> ASMKNCVIVSAVRTAIGSFNGSLASTSAIDLGATVIKAAIERAKIDSQ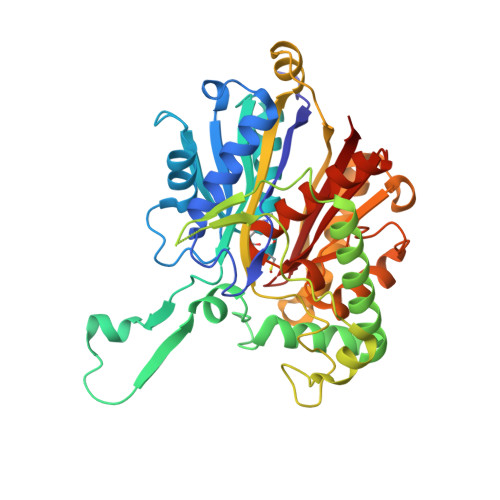HVDEVIMGNVLQAGLGQNPARQALLKSGLAETVCGFTVNKVCGSGLKSVALAAQAIQAGQAQSIVAGGMENMSLAPYLLDAKARSGYRLGDGQVYDVILRDGLMCATHGYHMGITAENVAKEYGITREMQDELALHSQRKAAAAIESGAFTAEIVPVNVVTRKKTFVFSQDEFPKANSTAEALGALRPAFDKAGTVTAGNASGINDGAAALVIMEESAALAAGLTPLARIKSYASGGVPPALMGMGPVPATQKALQLAGLQLADIDLIEANEAFAAQFLAVGKNLGFDSEKVNVNGGAIALGHPIGASGARILVTLLHAMQARDKTLGLATLCIGGGQGIAMVIERL>[2x]MNPAAEAEFNILLATDSYKVTHYKQYPPNTSKVYSYFECREKKTENSKLRKVKYEETVFYGLQYILNKYLKGKVVTKEKIQEAKDVYKEHFQDDVFNEKGWNYILEKYDGHLPIEIKAVPEGFVIPRGNVLFTVENTDPECYWLTNWIETILVQSWYPITVATNSREQKKILAKYLLETSGNLDGLEYKLRDFGYRGVSSQETAGIGASAHLVNFKGTDTVAGLALIKKYYGTKDPVPGYSVPAAEHSTITAWGKDHEKDAFEHIVTQFSSVPVSVVSDSYDIYNACEKIWGEDLRHLIVSRSTQAPLIIRPDSGNPLDTVLKVLEILGKKFPVTENSKGYKLLPPYLRVIQGDGVDINTLQEIVEGMKQKMWSIENIAFGSGGGLLQKLTRDLLNCSFKCSYVVTNGLGINVFKDPVADPNKRSKKGRLSLHRTPAGNFVTLEEGKGDLEEYGQDLLHTVFKNGKVTKSYSFDEIRKNAQLNIELEAAHHLEHHHHHHHH

NAMPT functions as a homo-dimeric enzyme that catalyzes the rate limiting step in the primary salvage pathway for NAD synthesis, the transfer of a phosphoribosyl residue from 5-phosphoribosyl-1-pyrophosphate (PRPP) to nicotinamide (NAM) to produce nicotinamide mononucleotide (NMN). Crystal structures of NAMPT in numerous ligand-bound forms have been reported. These structures consistently display a NAMPT homo-dimer with two essentially identical active sites at the dimer interface. Typical NAMPT inhibitors were found to occupy the portion of active site responsible for NAM binding and a tunnel-shaped cavity extending from the NAM binding site. Furthermore, we determine the crystal structures of six NAMPT mutants in the apo form and in complex with various inhibitors and present a definitive model to explain the differential effects of the mutations on various structural classes of NAMPT inhibitors.

H191 and G217 together with D219 and Y188 form one side of the tunnel wall surrounding the cavity commonly occupied by NAMPT inhibitors. A previously published in silico model predicted that H191R would protrude its side chain into the tunnel and sterically block inhibitors like APO866 from binding. When tested across a panel of structurally diverse inhibitors, H191R reduced potency across the compound families, but remained more sensitive to APO866 and GMX1778 than series A inhibitors. To reconcile the discrepancy, we determined the crystal structure of NAMPT-H191R. The R191 side chain indeed occupied part of the volume inside the tunnel region, but did not completely block the tunnel passage, thus imposing a more stringent limit on the size of linker moieties in the inhibitor molecules. The bi-aryl sulfone group of series A compounds exceeded the available space, whereas the more flexible and narrower linker of APO866 can fit through the altered tunnel. The H191R and all G217 mutant NAMPT proteins exhibited at least 100- fold increases in GNE-618 IC50 compared to wild-type.>[2x]ETGCNKALCASDVSKCLIQELCQCRPGEGNCSCCKECMLCLGALWDECCDCVGMCNPRNYSDTPPTSKSTVEELHEPIPSLFRALTEGDTQLNWNIVSFPVAEELSHHENLVSFLETVNQPHHQNVSVPSNNVHAPYSSDKEHMCTVVYFDDCMSIHQCKISCESMGASKYRWFHNACCECIGPECIDYGSKTVKCMNCMFGTKHHHHHH

Twisted gastrulation (TWSG1) is an evolutionarily conserved secreted glycoprotein which controls signaling by Bone Morphogenetic Proteins (BMPs). TWSG1 binds BMPs and their antagonist Chordin to control BMP signaling during embryonic development, kidney regeneration and cancer. TWSG1 is composed of two distinct, disulfide-rich domains. The TWSG1 N-terminal domain occupies the BMP type 1 receptor binding site on BMPs, whereas the C-terminal domain binds to a Chordin family member.

We crystallized and determined the TWSG1 structure at 2.6 Å resolution using a platinum single-wavelength anomalous diffraction experiment. TWSG1 crystallized as a dimer in the asymmetric unit, an arrangement that we observed in two crystal forms. The structure of TWSG1 reveals a modular architecture, comprising an α-helical N-terminal domain (NTD, Cys26–Arg80) connected by an extended 18 Å-long linker to a mixed-α/β C-terminal domain (CTD, Pro87–Phe223). The NTD of TWSG1 folds into a compact bundle of three α-helices locked by 7 disulfides. The CTD of TWSG1 is stabilized by 5 disulfide bonds (VIII–XII) and contains a sheet comprised of 5 antiparallel β-strands which constitute its core.>AATDISGAFEYSGWENFHRTQWSWDKKTRGAHLVNCTGACPHFVYSKDGVVMREEQSKDIAPMPNIPEYNPRGCNKGECGHDYMYGPHRIKYPLIRVGERGEGKWRRATWEEALDMIADKCVDTIKNHAPDCISVYSPVPAVSPVSFSAGHRFAHYIGAHAHTFYDWYGDHPTGQTQTCGVQGDTCETADWFNSKYIILWGSNPTQTRIPDAHFLSEAQLNGAKIVSISPDYNSSTIKVDKWIHPQPGTDGALAMAMAHVIIKEKLYDAHSLKEQTDLSYLVRSDTKRFLREADVVAGGSKDKFYFWNAKTGKPVIPKGSWGDQPEKKGSPVGFLGRNTFAFPKGYIDLGDLDPALEGKFNMQLLDGKTVEVRPVFEILKSRLMADNTPEKAAKITGVTAKAITELAREFATAKPSMIICGGGTQHWYYSDVLLRAMHLLTALTGTEGTNGGGMNHYIGQWKPAFVAGLVALAFPEGVNKQRFCQTTIWTYIHAEVNDEIISSDIDTEKYLRDSITTGQMPNMPEQGRDPKVFFVYRGNWLNQAKGQKYVLENLWPKLELIVDINIRMDSTALYSDVVLPSAHWYEKLDLNVTSEHSYINMTEPAIKPMWESKTDWQIFLALAKRVEMAAKRKKYEKFNDEKFKWVRDLSNLWNQMTMDGKLAEDEAAAQYILDNAPQSKGITIQMLREKPQRFKSNWTSPLKEGVPYTPFQYFVVDKKPWPTLTGRQQFYLDHDTFFDMGVELPTYKAPIDADKYPFRFNSPHSRHSVHSTFKDNVLMLRLQRGGPSIEMSPLDAKPLGIKDNDWVEAWNNHGKVICRVKIRNGEQRGRVSMWHCPELYMDLLTGGSQSVCPVRINPTNLVGNYGHLFFRPNYYGPAGSQRDVRVNVKRYIGATPISF[3x];>[3x]MANVMKAPRRQLTYVTDLNKCIGCQTCTVACKKLWTTGPGQDFMYWRNVETAPGLGYPRNWQTKGGGYKNGELQKGKIPPMIDYGIPFEFDYAGRLFEGKPGRVRPSPTPRSAPNWDEDQGAGEYPNNSFFYLPRMCNHCTKPACLEACPNEAIYKREQDGIVVIHQDKCKGAQACVQSCPYAKPYFNPLTNKANKCIGCFPRIEQGVAPACVAQCVGRAMHVGFVDDVNSSVYKLIKQYKVALPLHPEFGTEPNVFYVPPVLGPRIEMANGEPSTDPKIPLAQLEGLFGKQVR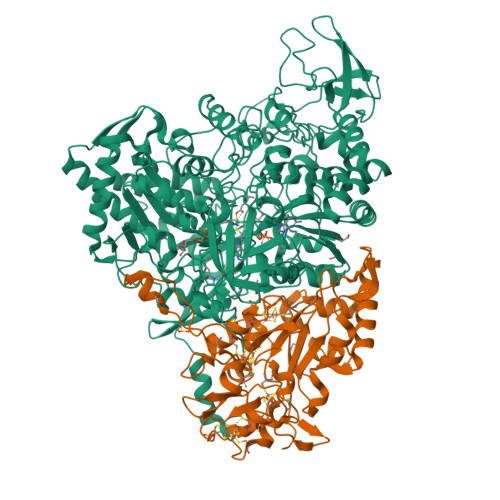DVLAILQSEREKKMKGLASDLMDVLIGRRSTDMMISPLT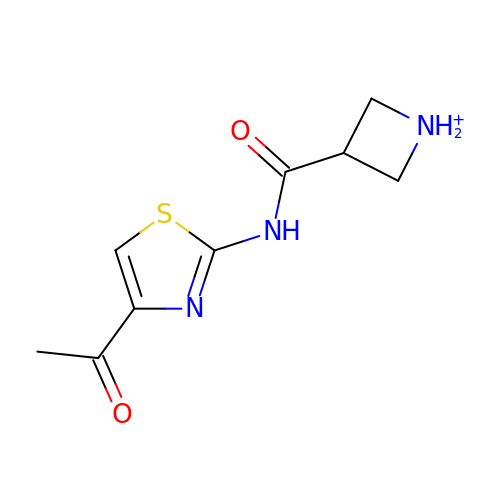~{N}-(4-ethanoyl-1,3-thiazol-2-yl)azetidin-1-ium-3-carboxamide | C9 H12 N3 O2 S | HHOKILYJEJQQMO-UHFFFAOYSA-O> MWNPIVNVDITLNTAGTTREGFGLPLFLASTDNFEERIRGYTSLTEVAEDFDESTAAYKAAKQLWSQTPKVTQLYIGRRTMQYTVSIPDTVAEGSEYSLTVAIGGGVSQPFQYTAKENDTALIVLNEFKSQIEASPTIKDGVNASVTGTGASATMIITKAGDNDFVKVTSITPTTSIAATTADTASAALASIETYSTDWYFISAEDRTQQFVLAMASEIQARKKIFFTANADVKALQGTDLTSATDVPAQLAKSKYTRTVCLWHHTAEFDYPEMAYIAYGAPYDAGSIAWGNAQLTGVAASLQPANQRPLISIQKSALDTRSCNFIDLDGGVPVVRRGITSGGEWIDIVRGVDWLESDLKTSLRDLLINQKGGKITYDDTGITRIRQVIETSLQRAVNRKFLSTYTVTVPKASQVALADKKARILKDITFHGILAGAILDVDLKGTVAYE;> MAMYQQYSPKDVVCSWNGIAIEGFAPDSFLRLQRTSPLVTPVVGAGGQVALTRNADKTGTIEIELMQTSLSNQMLSAIQAKQDDMELEEDISSNFVIYDPSGSVLATGINAWLQELPQIELGRDQNSKTWIFGCEKLDYTSTIPASSV

Bacteriophage Sf14 infects the human pathogen Shigella flexneri. Here, we report multiple high-resolution structures of the full Sf14 particle, including symmetric and asymmetric reconstructions of the virion capsid, empty capsid, portal region, tail, and baseplate. Sf14 virions have a spherical icosahedral capsid of 820 Å in diameter, which is connected to a long, contractile tail that is approximately 1205 Å long and an average of 235 Å in diameter, expanding to 315 Å at the baseplate. Overall, phage Sf14 appears to share some similarities to other model phages, but in different combinations: both λ- and T4-like decoration proteins, HK97-like capsid and portal proteins, T4/Mu-like tail fibers, a Mu-like baseplate, and a P2-like tail needle.

Here we determined the full structure of the uncontracted, pre-ejection tail, including the tail fiber proteins, baseplate, and central tail needle. A helical reconstruction of the tail is shown in Fig. 6A, with cross-sections showing poorly resolved density in the central tube that could be attributed to tape measure proteins and/or genomic DNA. Dimers of the tail sheath and tube proteins (gp39 and gp40) that comprise the helix were also determined by ModelAngelo.> NEAIECHLSDLLQQLTSVNASKPSERGLVRQEEAEDPACIPIFWVSKWVDYSDKYGLGYQLCDNSVGVLFNDSTRLILYNDGDSLQYIERDGTESYLTVSSHPNSLMKKITLLNYFRNYMSEHLLKAGANITPREGDELARLPYLRTWFRTRSAIILHLSNGTVQINFFQDHTKLILCPLMAAVTYINEKRDFQTYRLSLLEEYGCCKELASRLRYARTMVDKLLSSRSASNRLKAS;> SPLVTSTIKTED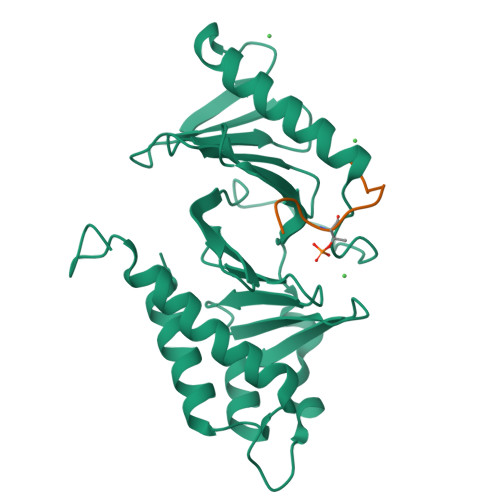VVSNSQNSRLHFSQHKTSTI> MDDESNAYLGTGWGFPPTFEKKARSVRLVSAEDDIRESLQILLST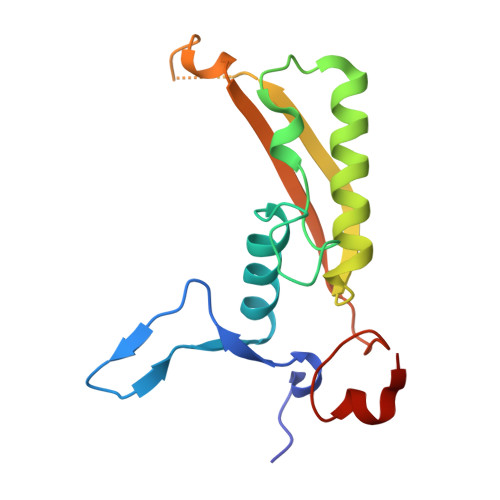NLGERVMQPNYGCNLQDLLFESLSPTVASNIKELVRTAILYYEPRIRLNKLDIQQGISDRQNPSAVNEADAQGLIQIIVDCTIISTNSRFNFVYPFYLQEGSGN>[2x]MAGNSIGQLFRVTTCGESHGVG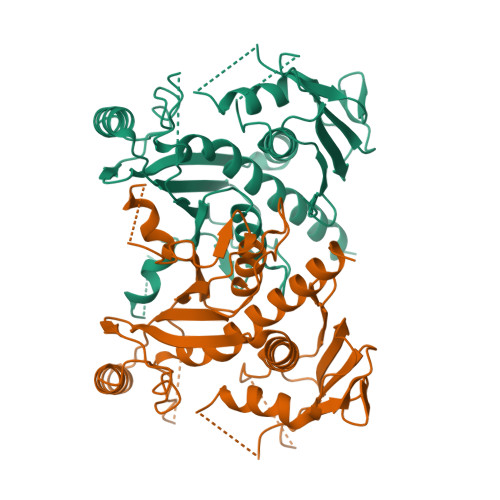LMAIVDGVPPGLALTEEDLQKDLDRRKPGTSKFATQRKEPDQVEIISGVFEGKTTGTPIGLLIRNTDQKSKDYGNIAQTFRPGHADYTYTQKYGFRDYRGGGRSSARETAMRVAAGAIAKKYLAEKFGVLIRGHVTQIGNEVAEKLDWNEVPNNPFFCGDVDAVPRFEALVTSLREQGTSCGAKLEILAEKVPVGWGEPVFDRLDADIAHAMMSINAVKGVEIGDGFAVAGQFGHETRDELTSHGFLANHAGGILGGISSGQTIRVAIALKPTASITTPGKTINLNREDTDVLTKGRHDPCVGVRATPIAEAMLAIVLMDHFLRHRAQNADVVPPFAPIEP>[8x]GSMPRSSEGPLTGKVAFITGAARGQGRAHAVRLAADGADIIAVDLCDQIASVPYPLATPEELAATVKLVEDIGSRIVARQADVRDRESLSAALQAGLDELGRLDIVVANAGIAPMSAGDDGWHDVIDV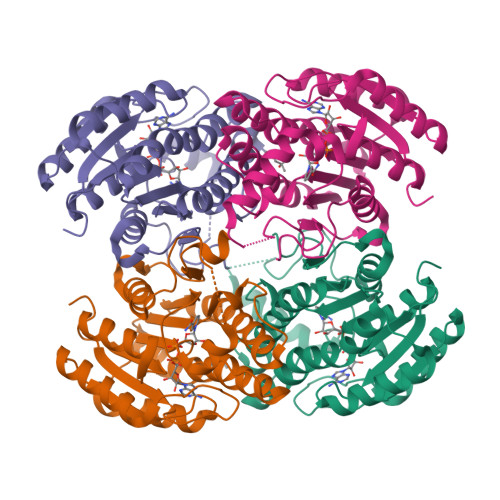NLTGVYHTIKVAIPTLVKQGTGGSIVLISSSAGLAGVGSADPGSVGYVAAKHGVVGLMRVYANLLAGQMIRVNSIHPSGVETPMINNEFTREWLAKMAAATDTPGAMGNAMPVEVLAPEDVANAVAWLVSDQARYITGVTLPVDAGFLNK>MFEARLVQGSILKKVLEALKDLINEACWDISSSGVNLQSMDSSHVSLVQLTLRSEGFDTYRCDRNLAMGVNLTSMSKILKCAGNEDIITLRAEDNADTLALVFEAPNQEKVSDYEMKLMDLDVEQLGIPEQEYSCVVKMPSGEFARICRDLSHIGDAVVISCAKDGVKFSASGELGNGNIKLSQTSNVDKEEEAVTIEMNEPVQLTFALRYLNFFTKAT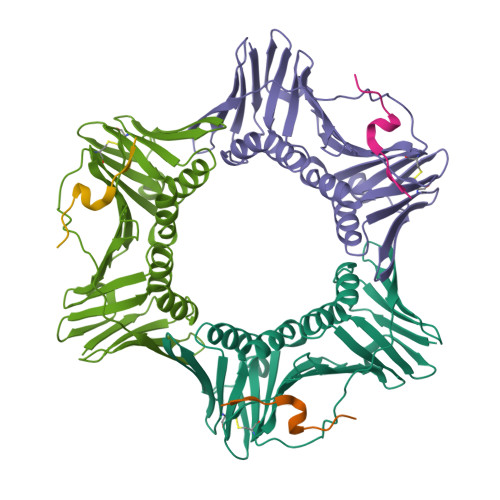PLSSTVTLSMSADVPLVVEYKIADMGHLKYYLAPKIEDEE[3x];>[3x]KRRQTSMTDYYHSKR> GSHMDELAPPKPPLPEGEVPPPRPPPPEEKDEEFPEQKAGEVINQPMMMAARQLHDEARKWSSKPGIPAAEVGIGVVAEADAADAAGFPVPPDMEDDYEPELLLMPSNQPVNQPILAAAQSLHREATKWSSKGNDIIAAAKRMALLMAEMSRLVRGGSGTKRALIQCAKDIAKASDEVTRLAKEVAKQCTDKRIRTNLLQVCERIPTISTQLKILSTVKATMLGRTNISDEESEQATEMLVHNAQNLMQSVKETVREA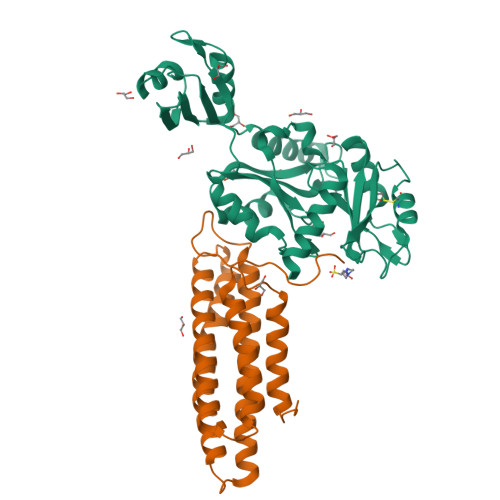EAASIKIRTDAGFTLRWVRKTPWYQ;> HMLDPEEIRKRLEHTERQFRNRRKILIRGLPGDVTNQEVHDLLSDYELKYCFVDKYKGTAFVTLLNGEQAEAAINAFHQSRLRERELSVQLQPTDALLCVANLPPSLTQQQFEELVRPFGSLERCFLVYSERTGQSKGYGFAEYMKKDSAARAKSDLLGKPLGPRTLYVHWTDAGQLTPALLHSRCLCVDRLPPGFNDVDALCRALSAVHSPTFCQLACGQDGQLKGFAVLEYETAEMAEEAQQQADGLSLGGSHLRVSFCAPGPPGRSMLAALIAAQATALNRG> TMAHHHHHHHHHGIEGRMSQDTEVDMKEVELNELEPEKQPMNAASGAAMSLAGAEKNGLVKIKVAEDEAEAAAAAKFTGLSKEELLKVAGSPGWVRTRWALLLLFWLGWLGMLAGAVVIIVRAPRCRELPAQKWWHTGALYRIGDLQAFQGHGAGNLAGLKGRLDYLSSLKVKGLVLGPIHKNQKDDVAQTDLLQIDPNFGSKEDFDSLLQSAKKKSIRVILDLTPNYRGENSWFSTQVDTVATKVKDALEFWLQAGVDGFQVRDIENLKDASSFLAEWQNITKGFSEDRLLIAGTNSSDLQQILSLLESNKDLLLTSSYLSDSGSTGEHTKSLVTQYLNATGNRWCSWSLSQARLLTSFLPAQLLRLYQLMLFTLPGTPVFSYGDEIGLDAAALPGQPMEAPVMLWDESSFPDIPGAVSANMTVKGQSEDPGSLLSLFRRLSDQRSKERSLLHGDFHAFSAGPGLFSYIRHWDQNERFLVVLNFGDVGLSAGLQASDLPASAS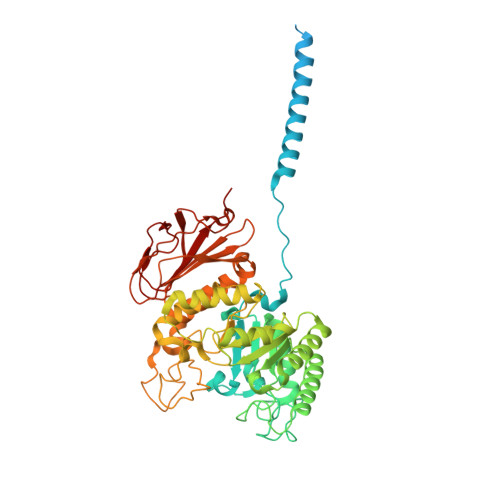LPAKADLLLSTQPGREEGSPLELERLKLEPHEGLLLRFPYAA2-(1,3,5-trimethyl-1H-pyrazol-4-yl)ethanol 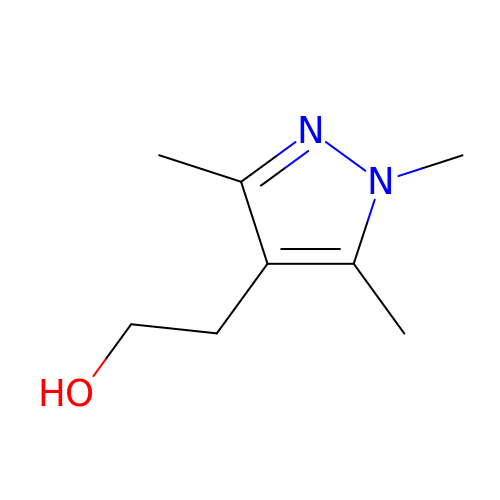| C8 H14 N2 O | QESMYIFDOLAREQ-UHFFFAOYSA-N> GPLGSIRVMLIDDHPVVRAGLRSILDSFDDITVVAEASDGSNINTKGIDVVVTDIQMPGTDGITLTRALANAGGPPVLILTTYDTEADILAAVEAGAMGYLLKD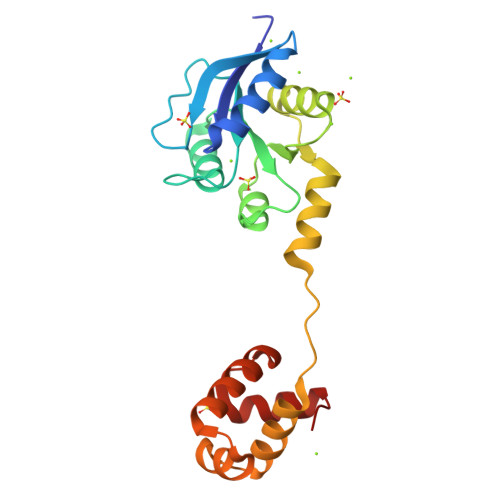APESALHDAVVATFEGRRTLAPEVANALMQRVSKPRQALSAREIEILQNLEQGLSNRQLAAKLFISEATVKTHLVHIYSKLGVDNRTAAITAARQQRLI> AAVTQSPRNKVAVTGEKVTLSCQQTNNHNNMYWYRQDTGHGLRLIHYSYGAGSTEKGDIPDGYKASRPSQEQFSLILESATPSQTSVYFCASGGGGTLYFGAGTRLSVL;> ESQPDPMPDDLHKSSEFTGTMGNMKYLYDDHYVSATKVKSVDKFLAHDLIYNISDKKLKNYDKVKTELLNEDLAKKYKDEVVDVYGSNYYVNCYFSSKDNVWWPGKTCMYGGITKHEGNHFDNGNLQNVLVRVYENKRNTISFEVQTDKKSVTAQELDIKARNFLINKKNLYEFNSSPYETGYIKFIENNGNTFWYDMMPAPGDKFDQSKYLMM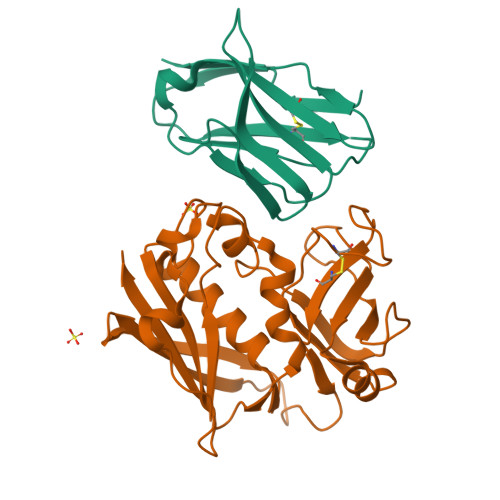YNDNKTVDSKSVKIEVHLTTKNG> AKMAFTLADRVTEEMLADKAALVVEVVEENYHAAPIVGIAVVNEHGRFFLRPETALADPQFVAWLGDETKKKSMFDSKRAAVALKWKGIELCGVSFDLLLAAYLLDPAQGVDDVAAAAKMKQYEAVRPDEAVYGKGAKRAVPDEPVLAEHLVRKAAAIWALERPFLDELRRNEQDRLLVELEQPLSSILAEMEF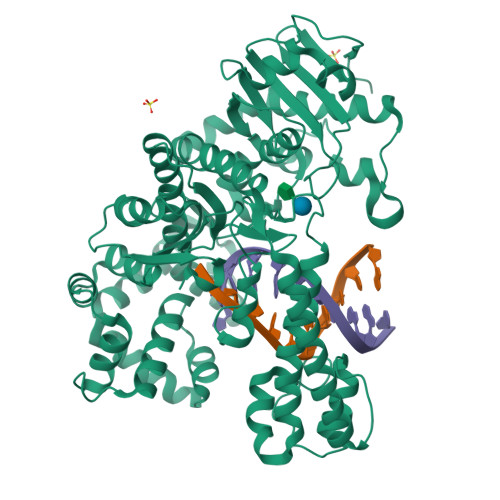AGVKVDTKRLEQMGEELAEQLRTVEQRIYELAGQEFNINSPKQLGVILFEKLQLPVLKKSKTGYSTSADVLEKLAPYHEIVENILHYRQLGKLQSTYIEGLLKVVRPDTKKVHTIFNQALTQTGRLSSTEPNLQNIPIRLEEGRKIRQAFVPSESDWLIFAADYSQIELRVLAHIAEDDNLMEAFRRDLDIHTKTAMDIFQVSEDEVTPNMRRQAKAVNFGIVYGISDYGLAQNLNISRKEAAEFIERYFESFPGVKRYMENIVQEAKQKGYVTTLLHRRRYLPDITSRNFNVRSFAERMAMNTPIQGSAADIIKKAMIDLNARLKEERLQARLLLQVHDELILEAPKEEMERLCRLVPEVMEQAVTLRVPLKVDYHYGSTWYDAK>[4x]SMTIRFHRNDLPNLDNYQVDAVAIDTETLGLNPHRDRLCVVQISPGDGTADVIQIEAGQKKAPNLVKLLKDRSITKIFHFGRFDLAVLAHAFGTMPQPVFCTKIASKLTRTYTDRHGLKEICSELLDVSISKQQQSSDWAAEVLSQAQLEYAASDVLYLHRLKAVLEQRLERDGRTKQAEACFKFLPTRSELDLMGWAESDIFAHS

Orn and NrnC are 3′–5′ exonucleases with a DnaQ fold containing the catalytic DEDD motif, a domain that is common in enzymes that act on nucleic acids. Notably, Orn (and its eukaryotic ortholog REXO2) or NrnC activity is critical for cellular growth, rendering them unique amongst the exoribonucleases known to date. Through quantitative structure-function analyses, we show here that NrnC-type RNases share this narrow substrate length preference with Orn. The structures confirm an octameric assembly as a conserved feature of NrnC-type RNases.

To further understand the structural basis of NrnC’s substrate preference, we determined structures of B. melitensis NrnC (NrnCBm) in several apo and partially pGG-bound states. (C) Superposition of four apo-NrnCBm conformations based on three independent crystal forms (comprising chains apo1A/apo1B for form 1; apo2A/apo2B for form 2, and apo3A/pGG-bound3B for form 3), compared to the pGG-bound conformation of the same protein shown in (B). In a second apo-NrnCBm crystal form, we captured an alternate conformation in which the conserved hydrophobic residue F79 moves into the active site. The movement of this residue, which is adjacent to the phosphate cap residue H78, is realized through a flip of the peptide backbone and would introduce a clash with the nucleotide. In the same structure, the flexible SKQQQS loop is collapsed into the active site, trapping the catalytic residue Y150 in an intermediate conformation, which would introduce further clashes with the nucleotide substrate. Simultaneously, a rotamer change of the phosphate-cap residue H204 pivots its sidechain away from the active site, opening it for access to substrates. This conformation may depict a post-hydrolysis state, suggesting a mechanism for product release.>GHMINYPLASSTWDDLEYKAIQSVLDSKMFTMGEYVKQYETQFAKTFGSKYAVMVSSGSTANLLMIAALFFTKKPRLKKGDEIIVPAVSWSTTYYPLQQYGLRVKFVDIDINTLNIDIESLKEAVTDSTKAILTVNLLGNPNNFDEINKIIGGRDIILLEDNCESMGATFNNKCAGTFGLMGTFSSFYSNHIATMEGGCIVTDDEEIYHILLCIRAHGWTRNLPKKNKVTGVKSDDQFEESFKFVLPGYNVRPLEMSGAIGIEQLKKLPRFISVRRKNAEYFLDKFKDHPYLDVQQETGESSWFGFSFIIKKDSGVIRKQLVENLNSAGIEC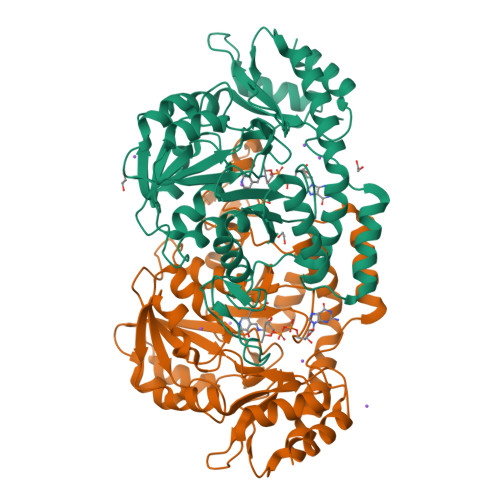RPIVTGNFLKNTDVLKYFDYTVHNNVDNAEYLDKNGLFVGNHQIELFDEIDYLREVLK[2x]>ADLYENPMGLMGFEFI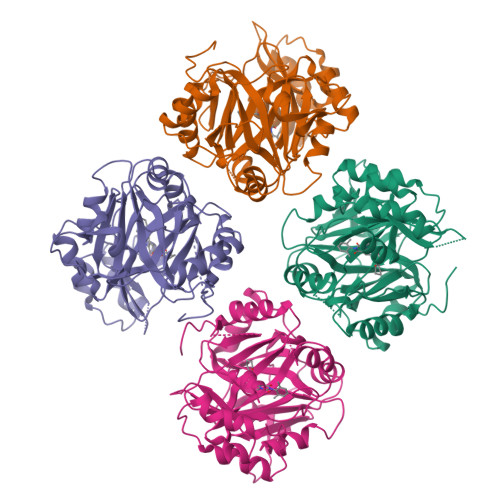EFASPTPGTLEPIFEIMGFTKVATHRSKNVHLYRQGEINLILNNEPNSIASYFAAEHGPSVCGMAFRVKDSQKAYNRALELGAQPIHIDTGPMELNLPAIKGIGGAPLYLIDRFGEGSSIYDIDFVYLEGVERNPVGAGLKVIDHLTHNVYRGRMVYWANFYEKLFNFREARYFDIKGEYTGLTSKAMSAPDGMIRIPLNEESSKGAGQIEEFLMQFNGEGIQHVAFLTDDLVKTWDALKKIGMRFMTAPPDTYYEMLEGRLPDHGEPVDQLQARGILLDGSSVEGDKRLLLQIFSETLMGPVFFEFIQRKGDDGFGEGNFKALFESIERDQVRRGVLATD[4x]Here, we show that Pseudomonas aeruginosa OprC is an outer membrane, TonB-dependent transporter that is conserved in many Proteobacteria and which mediates acquisition of both reduced and oxidised ionic copper via an unprecedented CxxxM-HxM metal binding site. As indicated by the successful structure solution, OprC contains a single bound copper and shows the typical fold of a TBDT, with a large 22-stranded β-barrel occluded by an N-terminal approximately 15 kDa plug domain that, like in other TBDTs, completely occludes the lumen of the barrel. The copper binding site comprises residues Cys143 and Met147 in the plug domain and His323 and Met325 in the barrel wall. The CxxxM-HxM configuration, which coordinates the copper in a tetrahedral manner, is highly unusual and has, to our knowledge, not been observed before in copper homeostasis proteins.

To obtain copper-free OprC after purification from rich media, we constructed a variant (OprCAA) in which the binding site residues Cys143 and Met147 were both mutated to alanines. Even after equilibration of OprCAA for 30 min with 3 or 10 equivalents Cu(II), no coelution with metal is observed, indicating that high-affinity copper binding is completely abolished and confirming that the His7 tag does not bind Cu(II) with an affinity high enough to survive SEC, possibly due to the presence of 0.5 mM EDTA in the SEC buffer. The OprCAA structure was solved by molecular replacement (MR) using Cu-bound OprCWT as the search model. The binding site residues of both structures occupy very similar positions, indicating that the introduced mutations abolish copper binding without generating gross changes in the binding site. Superposition of the structures shows that for the remainder of the protein, structural changes upon copper binding are confined to the vicinity of the copper binding site, with parts far removed virtually unchanged (overall Cα RMSD approximately 1.0 Å). The largest change is observed for loop L11, which undergoes an inward-directed motion of approximately 8.0 Å upon copper binding (S3D, S3E). Some loop tips (e.g., L4, L5, L6) in OprCAA lack electron density for a limited number of residues, suggesting increased mobility. In the double mutant, copper becomes solvent accessible due to the absence of the Met147 side chain (S3D, S3E). In OprCAA, N-terminal density is visible up to Leu66 (i.e., the first 10 residues of the mature protein are disordered) including the Ton box (68PSVVTGV75), which is tucked away against the plug domain and the barrel wall. The observed position of the Ton box in OprCAA, likely hard to reach from the periplasmic space, would prevent nonproductive interactions of TonB with transporters that do not have substrate bound.

>MEKRMSTQQRAAGNACPTAAFSFDPARLAQRRRWAGAFAALCGLALSPSALLAEEHSQHQDHAVELAPSVVTGVAQSSPLTIVTNPKEPRQPVPASDGADYLKTIPGFAVIRNGGSNGDPVLRGMFGSRLNILTNGGMMLGAAPNRADAPTSYISPETYDKLTVIKGPQTVLWGPGASAGTILFEREPERFGELGSRVNASLLAGSNGRFDKVLDAAAGNRLGYLRFTGNHAQSDDYEDGAGNTVPSRWKKWNGDVAVGWTPDEDTLIELTAGKGDGEARYAGRGMDGSQFKRESLGLRFVKSNVSDVLEKVEAQVYYNYADHIMDNFRLRTPDPSSMMPMPMASQVDRRTLGGRLAATWRWDDFKLVTGVDAMRNEHRARGSKYDMMTDYYTDADQFPWSKDAVFHNYGAFGELTWFAAERDRLIGGLRLDRASVKDYRQTLKSGHMGHAMANPTANDTRADTLPSGFVRYEHDLADSPTTLYAGLGHAERFPDYWELFSPKRGPNGSVNAFDKIKPEKTTQLDFGLQYNGDKLQAWASGYVGVVQDFILFSYREGMMGSSTQATNVDARIMGGELGASYQLTGNWKTDASLAYAWGKNSSDDRALPQIPPLEARFGLTYEEGDWSAGSLWRVVAPQNRIARDQGNVVGKDFDKSAGFGVFSLNGAYRVTRNVKLSAGVDNLFDKDYTEHLNKAGDAGFGFSANETVPEPGRTFWTKVDFSF[2x]(2R)-2-hydroxy-3-(1H-indol-3-yl)propanoic 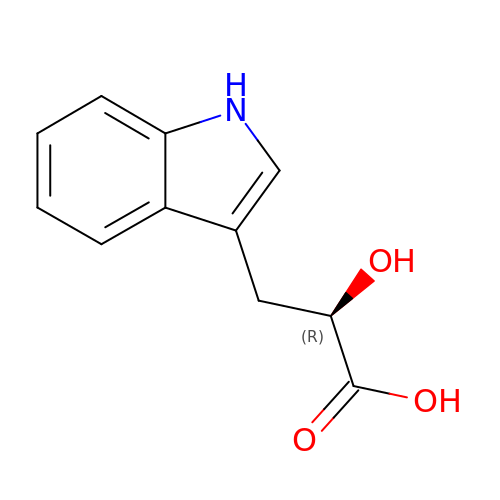acid | C11 H11 N O3 | XGILAAMKEQUXLS-SNVBAGLBSA-N2C-METHYL-D-ERYTHRITOL 2,4-CYCLODIPHOSPHATE | C5 H12 O9 P2 | 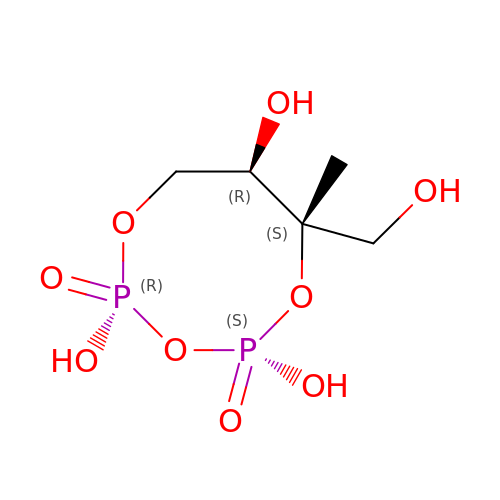SFRQRNJMIIUYDI-UHNVWZDZSA-N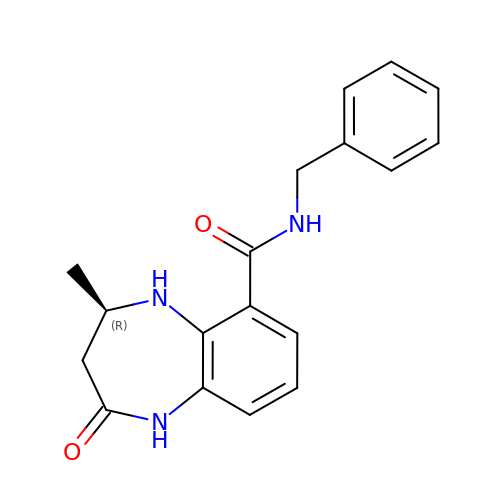(4R)-N-benzyl-4-methyl-2-oxo-2,3,4,5-tetrahydro-1H-1,5-benzodiazepine-6-carboxamide | C18 H19 N3 O2 | NUBAPEXWNUTLEU-GFCCVEGCSA-N> SSLPVPYKLPVSLSVGSCVIIKGTPIHSFINDPQLQVDFYTDMDEDSDIAFHFRVRFGNHVVMNRREFGIWMLEETTDYVPFEDGKQFELCIYVHYNEYEIKVNGIRIYGFVHRIPPSFVKMVQVSRDISLTSVCVCN

Galectin (Gal) is a lectin that binds to β-galactosides. Because the primary and tertiary structures of Gal-13 are highly conserved among all galectins, it had been named galectin-13. However, our crystallographic and biochemical experiments (solid phase experiment, hemagglutination assay, and biolayer interferometry) proved that wild-type Gal-13 could not bind lactose or a rhamnogalacturonan Ι domain (RG-I-4) from Ginseng Pectin. Primary structure alignment showed that a highly conserved histidine residue was modified to arginine (Arg53) in the ligand binding site of wild-type Gal-13, which may be why Gal-13 could not bind lactose.

All three other variants (R53HH57R, R53HR55NH57R, and R53HR55NR57RD33G) co-crystallized with lactose, but not Tris, even when the crystallization conditions contained 100 mM Tris. This indicates that these three variants prefer to binding lactose. Without this residue, Gal-13 cannot bind lactose. The present results showed that double mutation of R53 to H and H57 to R was sufficient to recover the ability of Gal-13 to bind lactose. Arg57 in R53HH57R and R53HH57RD33G showed two different conformations. Arg57 in one conformation could indirectly stabilize the pyran ring of galactose through a water molecule (W). In the crystal of wild-type Gal-13, Asp33 from one monomer occupies a large part of the ligand binding site of another. However, in the R53HH57R variant, lactose repealed the side chain of Asp33, making Asp33 adopt an awkward conformation. Variant R53HH57R demonstrated greater bio-activity (MAC: 6.25 µg/ml) than wild-type Gal-13, and all other variants had similar activities (25 or 12.5 µg/ml) as wild-type protein.[(2R)-2-{2-[hydroxy(methyl)amino]-2-oxoethyl}-5-phenylpentyl]phosphonic 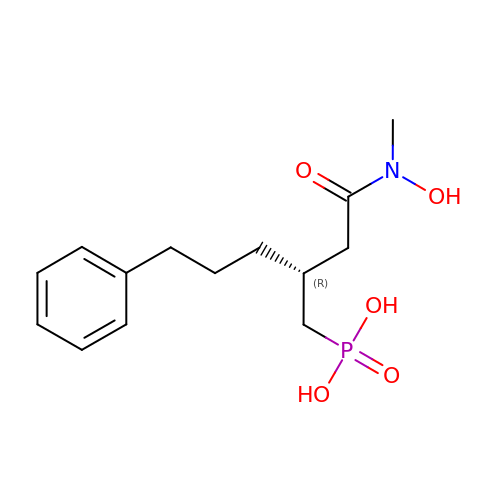acid | C14 H22 N O5 P | YKRNADVNYIPUET-CYBMUJFWSA-N> HIEVVGKLGSTYGIRGWLRIYSSTEQAES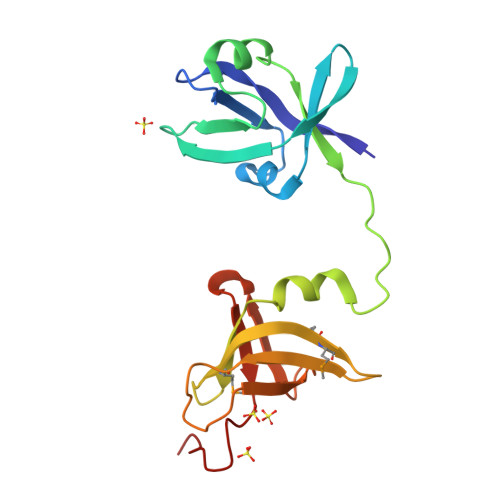IFDYQPWFLKIKGEWQSIELENWRYHNHEIIVKLKGVDDREAAQILANVEIGVDLSVFPELEEGDYYWHDLIGCTVVNLEGYTMGTVTEMMETGSNDVLVVKANTKDAFGKQERLIPFLYEQVVKRVDLTTKTIEVDWDAGFLEHHHH>MIIGYVIGQATTQEALILAERPVRLGTYVVLEYDNVKALGLITNVTRGSPLLDDNMNDIEIVQRLKQFNNSIPVYTKAKVKLLCDMNNHFLMPDIPPFAGTPAREAEDEELKSIYSQDGQIRIGSLIGKNVEVKLNINSFARHLAILAATGSGKSNTVAVLSQRISELGGSVLIFDYHGEYYDSDIKNLNRIEPKLNPLYMTPREFSTLLEIRENAIIQYRILRRAFIKVTNGIRAALAAGQIPFSTLNSQFYELMADALETQGNSDKKSSAKDEVLNKFEEFMDRYSNVIDLTSSDIIEKVKRGKVNVVSLTQLDEDSMDAVVSHYLRRILDSRKDFKRSKNSGLKFPIIAVIEEAHVFLSKNENTLTKYWA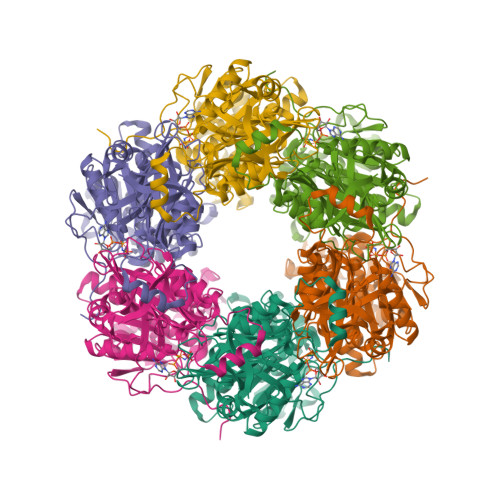SRIAREGRKFGVGLTIVSQRPKGLDENILSQMTNKIILKIIEPTDKKYILESSDNLSEDLAEQLSSLDVGEAIIIGKIVKLPAVVKIDMFEGKLLGSDPDMIGEWKKVAASEKIAKGFADFGTEIGD[2x]>[2x]MRRPDTPATPPPSAEPPGGVVVPPGTRKPRPEFQSADCPDVMMVSIPGTWESSPTDDPFNPTQFPLSLMSNISKPLAEQFGPDRLQVYTTPYTAQFHNPFAADKQMSYNDSRAEGMRTTVKAMTDMNDRCPLTSYVIAGF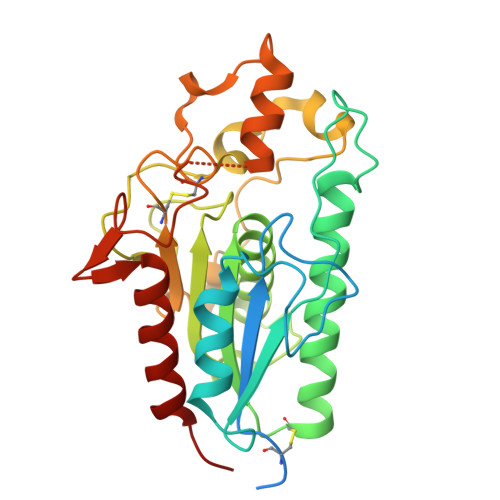SQGAVIAGDIASDIGNGRGPVDEDLVLGVTLIADGRRQMGVGQDVGPNPAGQGAEITLHEVPALSALGLTMTGPRPGGFGALDNRTNQICGSGDLICSAPEQAFSVFNLPKTLETLSGSAAGPVHALYNTPQFWVENGQTATQWTLEWARNLVENAPHPKHG>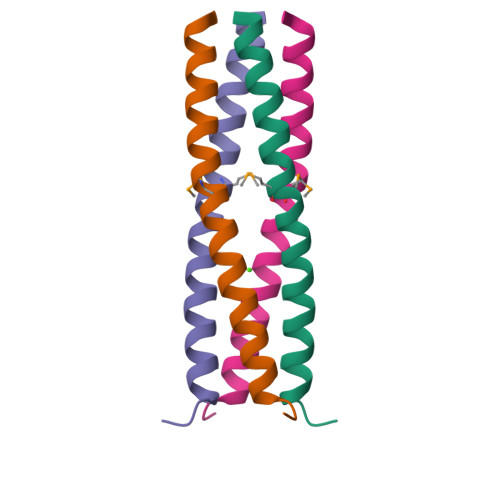[2x]IEKQMDRVVKEMRRQLEMIDKLTTREIEQVELLKRIYDKLTVQ> MPYHPALESLLDTPEIRKIKKLDLRDQRKIFADLSIAQIKRLPRPDIIEEDIKLENDTILRHYKPKKASDKAVLFIHGGGWCLSSIDTYDHVCRYLCDQGNLNIFSLEYGLGPEDKYPAAVNHALYAYDWLYENITKFNLS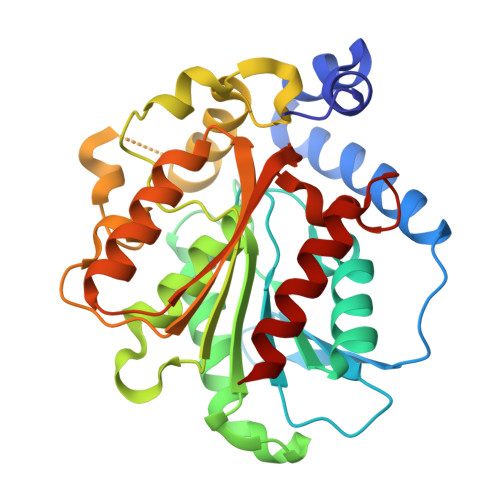TENIFVMGDSAGGNLVTIICHERQENMPKAQILVYPAVDMYTKYDSNTKFDEYKYHLTTEWCELFLKAYIGEDIMSEPKKLRQPTISPLFYKDTNQPDTLIVAATHDILIDGIYAYEEKLKQQGTYVETHYDDEMYHGFIGGLGVVPFENPKIALDKIIEFINKR P1-(5'-ADENOSYL)P5-(5'-(3'AZIDO-3'-DEOXYTHYMIDYL))PENTAPHOSPHATE 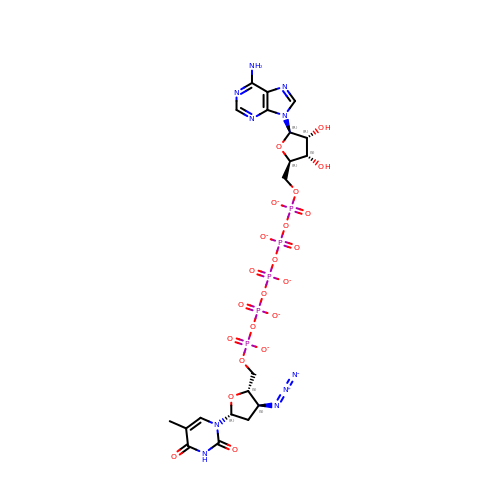| C20 H24 N10 O22 P5 | QNIWSXQXLJIUJW-SLFMBYJQSA-I>MSSLARGISRRRTEVATQVEAAPTGLRPNAVVGVRLAALADQVGAALAEGPAQRAVTEDRTVTGVTLRAQDVSPGDLFAALTGSTTHGARHVGDAIARGAVAVLTDPAGVAEIAGRAAVPVLVHPAPRGVLGGLAATVYGHPSERLTVIGITGTSGKTTTTYLVEAGLRAAGRVAGLIGTIGIRVGGADLPSALTTPEAPTLQAMLAAMVERGVDTVVMEVSSHALALGRVDGTRFAVGAFTNLSRDHLDFHPSMADYFEAKASLFDPDSALRARTAVVCIDDDAGRAMAARAADAITVSAADRPAHWRATDVAPTDAGGQQFTAIDPAGVGHHIGIRLPGRYNVANCLVALAILDTVGVSPEQAVPGLREIRVPGRLEQIDRGQGFLALVDYAHKPEALRSVLT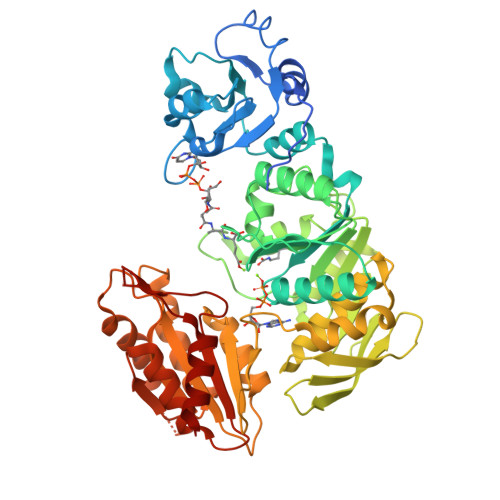TLAHPDRRLAVVFGAGGDRDPGKRAPMGRIAAQLADLVVVTDDNPRDEDPTAIRREILAGAAEVGGDAQVVEIADRRDAIRHAVAWARPGDVVLIAGKGHETGQRGGGRVRPFDDRVELAAALEALERRA[4x]>[7x]MIAELFTNNALNLVIIFGSCAALILMSFWFRRGNRKRKGFLFHAVQFLIYTIIISAVGSIINYVIENYKLKFITPGVIDFICTSLIAVILT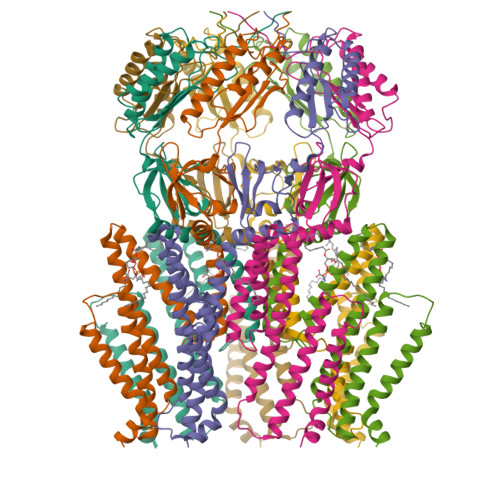IKLFLLINQFEKQQIKKGRDITSARIMSRIIKITIIVVLVLLYGEHFGMSLSGLLTFGGIGGLAVGMAGKDILSNFFSGIMLYFDRPFSIGDWIRSPDRNIEGTVAEIGWRITKITTFDNRPLYVPNSLFSSISVENPGRMTNRRITTTIGLRYEDAAKVGVIVEAVREMLKNHPAIDQRQTLLVYFNQFADSSLNIMVYCFTKTTVWAEWLAAQQDVYLKIIDIVQSHGADFAFPSQTLYMDNITPPEQGR The flagellar filament, a tubular structure composed of thousands of copies of the protein flagellin (FliC in many bacteria), exhibits helical symmetry in its straight non-motile forms and is supercoiled with a three-dimensional waveform in motile bacteria. Flagellar filaments can be neatly divided structurally into the two highly conserved inner domains, D0 and D1, which form the inner core of the filament, and a diverse number of outer domains, which decorate the inner core. Here we show that in the Pseudomonas aeruginosa PAO1 strain, a bacterium that forms a ridged filament with a dimerization of its flagellin outer domains, motility is categorically dependent on these flagellin outer domains. Moreover, a comprehensive network of intermolecular interactions connecting the inner domains to the outer domains, the outer domains to one another, and the outer domains back to the inner domain filament core, is required for motility.

We used the same method here to reconstruct the PAO1 flagellar filament to 5 Å resolution. Using the composite flagellin model, we built a model of the full PAO1 flagellar filament and then fit it into the density map. Due to not imposing helical symmetry on our reconstruction there, we observed an inherent curvature in the density map, arising from the supercoiling of the filaments, which was preserved in the refined model we built. Between conformations 1 and 2, domains D2 differ from each other by a displacement of about 4–6 Å and domains D3 differed by about 8–15 Å. One protofilament on the outer curve of the filament had all of its outer domains in a single conformation (gold protofilament). This unique protofilament constitutes a seam or discontinuity in the helical symmetry of the outer domains. The seam is generated by the two conformations 1 and 2 alternating along the 5-start helix. An outer domain in the PAO1 filament forms three interfaces. The conformational states adopted by the PAO1 B type flagellin result in the formation of a rigid flagellar filament structure with a seam on the outer curve of its supercoiled structure.

>VNTNIASLNTQRNLNASSNDLNTSLQRLTTGYRINSAKDDAAGLQISNRLSNQISGLNVATRNANDGISLAQTAEGALQQSTNILQRIRDLALQSANGSNSDADRAALQKEVAAQQAELTRISDTTTFGGRKLLDGSFGTTSFQVGSNAYETIDISLQNASASAIGSYQVGSNGAGTVASVAGTATASGIASGTVNLVGGGQVKNIAIAAGDSAKAIAEKMDGAIPNLSARARTVFTADVSGVTGGSLNFDVTVGSNTVSLAGVTSTQDLADQLNSNSSKLGITASINDKGVLTITSATGENVKFGAQTGTATAGQVAVKVQGSDGKFEAAAKNVVAAGTAATTTIVTGYVQLNSPTAYSVSGTGTQASQVFGNASAAQKSSVASVDISTADGAQNAIAVVDNALAAIDAQRADLAAVQNRFKNTIDNLTNISENATNARSRIKDTDFAAETAALSKNQVLQQAGTAILAQANQLPQAVLSLLR[33x]> MAH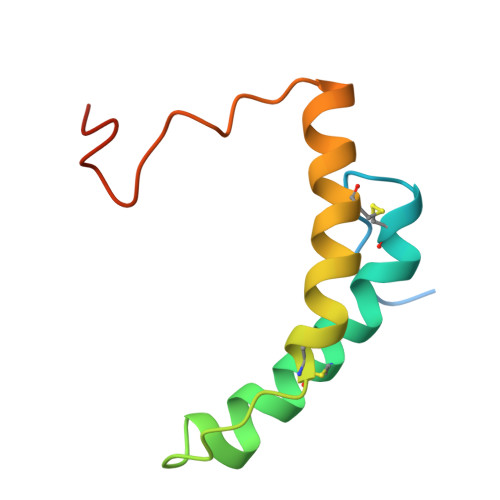HHHHHVDDDDKMNSVGEACTDMKREYDQCFNRWFAEKFLKGDSSGDPCTDLFKRYQQCVQKAIKEKEIPIEGLEFMGHGKEKPENSS>[2x]GSMNSNVENLPPHIIRLVYKEVTTLTADPPDGIKVFPNEEDLTDLQVTIEG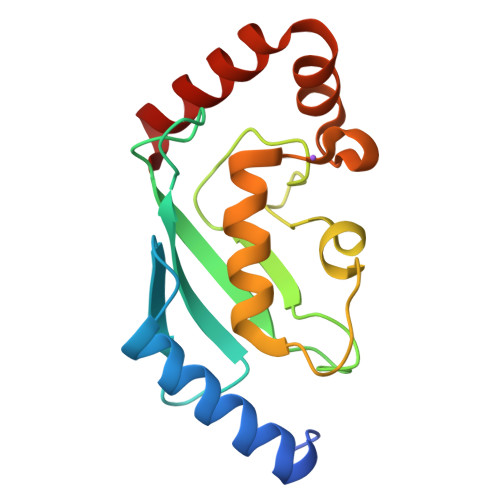PEGTPYAGGLFRMKLLLGKDFPASPPKGYFLTKIFHPNVGANGEICVNVLKRDWTAELGIRHVLLTIKCLLIHPNPESALNEEAGRLLLENYEEYAARARLLTEIHG Nicotinamide-N-methyltransferase (NNMT) is a cytosolic enzyme that catalyzes the transfer of a methyl group from S-adenosyl-methionine (SAM) to nicotinamide (Nam), yielding S-adenosyl-homocysteine (SAH) and 1-methylnicotinamide (MNam). NNMT is the major Nam-metabolizing enzyme, and systemic knockout in mice fully prevents MNam formation. As was described by Peng et al, NNMT possesses a class I AdoMet-dependent methyltransferase (MTase) core fold, comprising a central seven-stranded β-sheet, flanked on both sides by α-helices. In addition to the MTase core, there are two extra α-helices at the N-terminus, which, together with the β-hairpin Y203-S212, form a cap over the active site.

Based on the X-ray crystallographic data of our hits (1) and (2), the question arose as to whether the introduction of an appropriate 2-hydroxy-2-methyl-propionic carboxamide-based linker on (2) is able to transform our nicotinamide pocket binder into a true bisubstrate inhibitor. In our case, we saw the synthetic feasibility of transferring the corresponding structural motif directly to the imino nitrogen of compound delivering compound in the process. A subsequent X-ray analysis of confirmed the binding mode as a bisubstrate inhibitor. The binding mode in the SAH pocket of the part that is common between and is identical. The position of is slightly shifted with respect to the position of the tricyclic in, but also here the positions are very similar, showing that the fusion between the two inhibitor classes was successful. Further profiling on human and mouse NNMT enzyme revealed that a bisubstrate binding motif does not necessarily translate into an improved inhibitory activity. This may be related to the fact that a bisubstrate inhibitor has to compete with two substrates, SAM and Nam, which may be more difficult to achieve than when competing with a single substrate, especially when the second substrate, SAM, has a high affinity to the enzyme (Km = 1.8 µM, compared to 400 µM for Nam,). Based on our crystallographic data, we obtained the correct linker length allowing the important interactions with Val-143 and Tyr-204, and we also observed no obvious strains within the bound ligand. Our rational design towards the bisubstrate inhibitor starting from the fragment-sized nicotinamide pocket binder revealed no beneficial impact on in vitro inhibitory activity by addressing both binding sites of the NNMT enzyme simultaneously.

>MGSSHHHHHHSSGLVPRGSMESGFTSKDTYLSHFNPRDYLEKYYKFGSRHSAESQILKHLLKNLFKIFCLDGVKGDLLIDIGSGPTIYQLLSACESFKEIVVTDYSDQNLQELEKWLKAAPAAFDWSPVVTYVCDLEGNRVKGPEKEEKLRQAVKQVLKCDVTQSQPLGAVPLPPADCVLSTLCLDAACPDLPTYCRALRNLGSLLKPGGFLVIMDALKSSYYMIGEQKFSSLPLGREAVEAAVKEAGYTIEWFEVISQSYSSTMANNEGLFSLVARKLSRPL[4x]Besides 10–23 DNAzyme, 8–17 DNAzyme can also efficiently catalyze the cleavage reaction of RNA substrate, forming the 5′-product with a 2′,3′-cyclic phosphate at the 3′-end and the 3′-product with a hydroxyl group at the 5′-end; similar structural features are also observed on the cleavage products of the naturally occurred hammerhead, hairpin, and hepatitis delta virus (HDV) ribozymes. Interestingly, the same catalytic motif of 8–17 DNAzyme has been independently isolated under different selection conditions and using different cation cofactors, indicating that this small DNAzyme is efficient and its catalytic core motif is ubiquitous in the sequence space. The central catalytic core of 8–17 DNAzyme is flankedbytwo substrate-recognizing arms, which bind to the RNA substrate via the canonical Watson–Crick base pairing. The Dz36/substrate complexes assemble into a “V” shape with two arms (P1 and P2) orientated ~70° with respect to each other in all the three structures. Unexpectedly, the catalytic core forms a compact small DNA pseudoknot consisting of two short duplexes (P3 and P4) perpendicular to each other.

Crystals of one DNAzyme/native DNA complex and DNAzyme-(2′-OMe-G) were grown in the absence of PbCl2, whereas the crystals were grown in the presence of PbCl2 for another DNAzyme/native DNA complex structure, which captured one Pb2+ ion and is referred to as DNAzyme-Pb2+ hereafter. Among the three structures, DNAzyme-Pb2+ complex diffracted to the highest resolution (2.55 Å) and refinement resulted in a well-defined electron density for all the nucleotides. The DNAzyme-Pb2+ crystal adopts C2221 space group, it contains two Dz36-substrate complexes per asymmetric unit; each Dz36-substrate complex was clamped by two AsfvPolX molecules at the blunt ends. In the DNAzyme-Pb2+ complex structure, one Pb2+ ion was captured in the catalytic core. The Pb2+ ion coordinates with the O6 atom of G6, which forms G6:C12 pair identified structurally. Interestingly, the Pb2+ ion also coordinates with a water molecule interacting with the O5′ atom of G+1. While the distance between the Pb2+ and the water is 2.5 Å, the distance between the water and the O5′ atom of G+1 is 3.2 Å, indicating a hydrogen bond formation. This observation suggests that the 8–17 DNAzyme may catalyze the RNA cleavage reaction via the Pb2+ indirectly assisted mechanism and the Pb2+-coordinated water plays an important role in the catalysis. Besides orientating, coordination with the Pb2+ ion may also reduce the pKa of the water molecule; this water molecule may then serve as the general acid and provide a proton to the O5′ atom of G+1 for the O5′ leaving, thereby accelerating the RNA cleavage reaction. Due to the possible quick decay of the crystal and the dynamic binding with the DNAzyme, the occupancy (40%) of Pb2+ is not very high in our DNAzyme-Pb2+ structure.

>[4x]GGSMLTLIQGKKIVNHLRSRLAFEYNGQLIKILSKNIVAVGSLRREEKMLNDVDLLIIVPEKKLLKHVLPNIRIKGLSFSVKVCGERKCVLFIEWEKKTYQLDLFTALAEEKPYAIFHFTGPVSYLIRIRAALKKKNYKLNQYGLFKNQTLVPLKITTEKELIKELGFTYRIPKKRL> MASMTGGQQMGRGSMIFSVDKVRADFPVLSREVNGLPLAYLDSAASAQKPSQVIDAEAEFYRHGYAAVHRGIHTLSAQATEKMENVRKRASLFINARSAEELVFVRGTTAGINLVANSWGNSNVRAGDN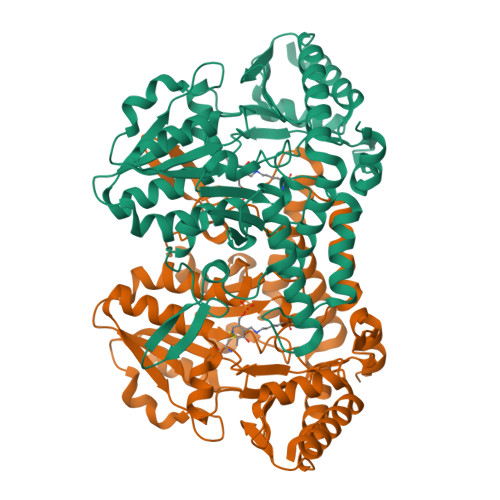IIISQMEHHANIVPWQMLCARVGAELRVIPLNPDGTLQLETLPTLFDEKTRLLAITHVSNVLGTENPLAEMITLAHQHGAKVLVDGAQAVMHHPVDVQALDCDFYVFSGHKLYGPTGIGILYVKEALLQEMPPWEGGGSMIATVSLSEGTTWTKAPWRFEAGTPNTGGIIGLGAALEYVSALGLNNIAEYEQNLMHYALSQLESVPDLTLYGPQNRLGVIAFNLGKHHAYDVGSFLDNYGIAVRTGHHCAMPLMAYYNVPAMCRASLAMYNTHEEVDRLVTGLQRIHRLLG>MGKSLSHLPLHSSKEDAYDGVTSENMRNGLVNSEVHNEDGRNGDVSQFPYVEFTGRDSVTCPTCQGTGRIPRGQENQLVALIPYSDQRLRPRRTKLYVMASVFVCLLLSGLAVFFLFPRSIDVKYIGVKSAYVSYDVQKRTIYLNITNTLNITNNNYYSVEVENITAQVQFSKTVIGKARLNNISIIGPLDMKQIDYTVPTVIAEEMSYMYDFCTLISIKVH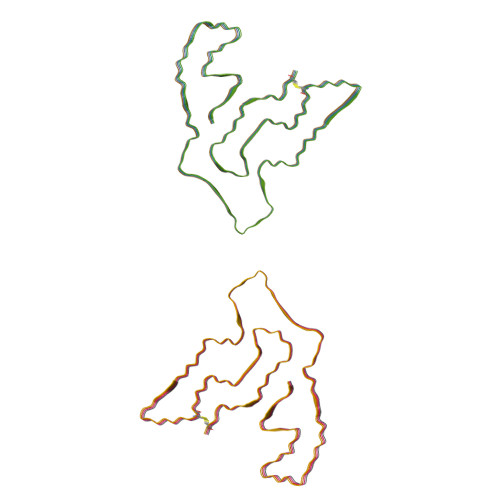NIVLMMQVTVTTTYFGHSEQISQERYQYVDCGRNTTYQLGQSEYLNVLQPQQ[8x]Usb1 is an exoribonuclease that shortens the oligo-uridine tail of U6 snRNA, resulting in a terminal 2′,3′ cyclic phosphate group in most eukaryotes, including humans. Usb1 is a member of the 2H phosphodiesterase superfamily, a large enzyme family containing members with known 2′,3′-cyclic or 1″,2″-cyclic phosphodiesterase (CPDase) activity, or 3′-5′ or 2′-5′ phosphodiesterase activity, or 2′,5′-RNA ligase activity. The active sites of 2H phosphodiesterase enzymes are characterized by a symmetric shape with two HxT/S motifs centered in a catalytic cleft. We report three high-resolution co-crystal structures of Usb1 complexed with RNA, which show the structural basis for this catalytic preference and unambiguously identify His120 and His208 as catalytic base and acid, respectively.

Mutation of His208 was found to confer the strongest defect in catalysis and was therefore used for crystallization trials, leading to successful structure determination of mutant Usb1 (H208Q) bound to RNA oligonucleotides 5′-UUUU-3′ and 5′-UUUA-3′. The RNAs are bound in the central cleft of Usb1. Only the last two nucleotides of RNA are clearly visible in the electron density maps, and the first two nucleotides are presumed to be disordered. The n–1 nucleotide binding pocket in both the H208Q-Usb1–UUUU and H208Q-Usb1–UUUA structures are nearly identical (r.m.s.d. = 0.3 Å). The structures show that His120 is positioned to function as a catalytic base by deprotonating the 2′ oxygen and facilitating an in-line attack on the scissile phosphodiester linkage. The n nucleotide binding pocket reveals the H208Q mutation that was used to generate the trapped Usb1–RNA complex forms hydrogen bonds with a non-bridging oxygen of the labile phosphodiester and the sidechain of Ser206 in both the UA and UU bound structures. Comparison of the wt-Usb1–AMP structure with the H208Q-Usb1–UUUA structure confirmed our hypothesis that the H208Q mutation perturbs the position of the scissile phosphate group and terminal nucleotide by ∼1 Å. In the H208Q structures, Ser210 is 3.7 Å away and cannot hydrogen bond to the phosphate group. For the H208Q Usb1 structures bound to UU and UA, both ribose sugar puckers on either side of the scissile phosphate are C2′ endo. Our observation that human Usb1 preferentially cleaves the dinucleotide UA is consistent with the hypothesis that the enzyme removes terminal adenosines from U6 snRNA in vivo, and provides a molecular explanation as to why U6 snRNAs from cells lacking Usb1 are adenylated.

> GAHMGNWATHVYVPYEAKEEFLDLLDVLLPHAQTYVPRLVRMKVFHLSLSQSVVLRHHWILPFVQALKARMTSFHRFFFTANQVKIYTNQEKTRTFIGLEVTSGHAQFLDLVSEVDRVMEEFNLTTFYQDPSFQLSLAWCVGDARLQLEGQCLQELQAIVDGFEDAEVLLRVHTEQVRCKSGNKFFSMPLK> MGISKTSSDLSEQLFQVSFVLARVLTSGIIMSIEKNENELKGL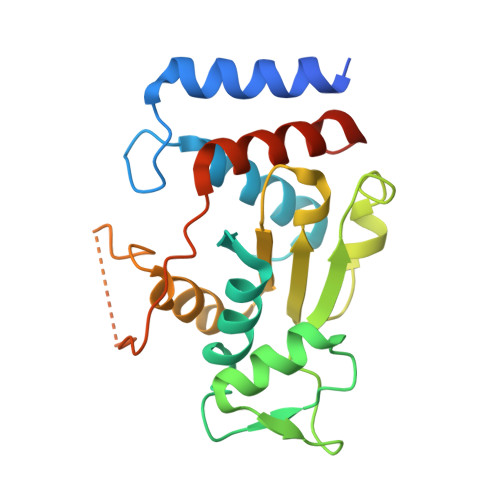ENILKKTSSKQYAVTFNSISGAVIGSLWGQDIVYGEATNQQSLDEQQEKLFKWLGIGHSSLLPEPYTLHAINWGNISNLQKITHEEAHVTLLDFTKLGFGPCAVLLTNNETIYKKSERLKIFGAFDLRTMWTQRETEKEIKPGLQFNFRLSPLVGACIKMALIKMGLNKHHHHHH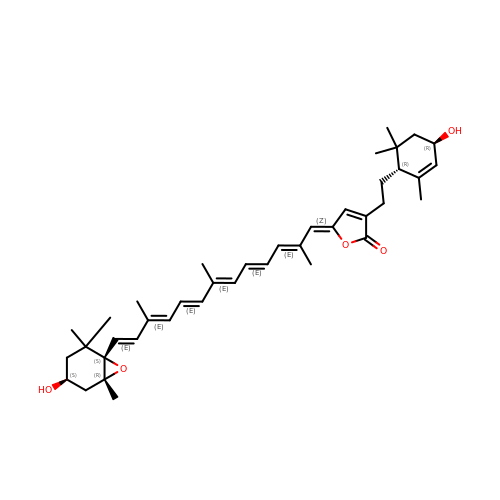(5~{Z})-3-[2-[(1~{R},4~{R})-2,6,6-trimethyl-4-oxidanyl-cyclohex-2-en-1-yl]ethyl]-5-[(2~{E},4~{E},6~{E},8~{E},10~{E},12~{E})-2,7,11-trimethyl-13-[(1~{S},4~{S},6~{R})-2,2,6-trimethyl-4-oxidanyl-7-oxabicyclo[4.1.0]heptan-1-yl]trideca-2,4,6,8,10,12-hexaenylidene]furan-2-one | C40 H54 O5 | JVBLPSSXRSHBAY-OQINAPANSA-N>[2x]MDWVIPPISVPENGKGPFPQRLVQLKSNKDRDTKIFYSITGPGADSPPEGVFAVEKETGWLLLN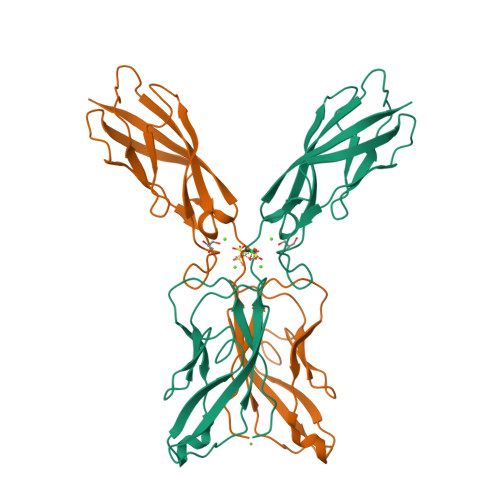KPLDREEIAKYELFGHAVSENGASVEDPMNISIIVTDQNDHKPKFTQDTFRGSVLEGVLPGTSVMQVTATDEDDAIYTYNGVVAYSIHSQEPKDPHDLMFTIHRSTGTISVISSGLDREKVPEYTLTIQATDMDGDGSTTTAVAVVEILD>[2x]YEQDKTYKITVLHTNDHHGHFWRNEYGEYGLAAQKTLVDGIRKEVAAEGGSVLLLSGGDINTGVPESDLQDAEPDFRGMNLVGYDAMAIGNHEFDNPLTVLRQQEKWAKFPLLSANIYQKSTGERLFKPWALFKRQDLKIAVIGLTTDDTAKIGNPEYFTDIEFRKPADEAKLVIQELQQTEKPDIIIAATHMGHYDNGEHGSNAPGDVEMARALPAGSLAMIVGGHSQDPVCMAAENKKQVDYVPGTPCKPDQQNGIWIVQAHEWGKYVGRADFEFRNGEMKMVNYQLIPVNLKKKVTWEDGKSERVLYTPEIAENQQMISLLSPFQNKGKAQLEVKIGETNGRLEGDRDKVRFVQTNMGRLILAAQMDRTGADFAVMSGGGIRDSIEAGDISYKNVLKVQPFGNVVVYADMTGKEVIDYLTAVAQMKPDSGAYPQFANVSFVAKDGKLNDLKIKGEPVDPAKTYRMATLNFNATGGDGYPRLDNKPGYVNTGFIDAEVLKA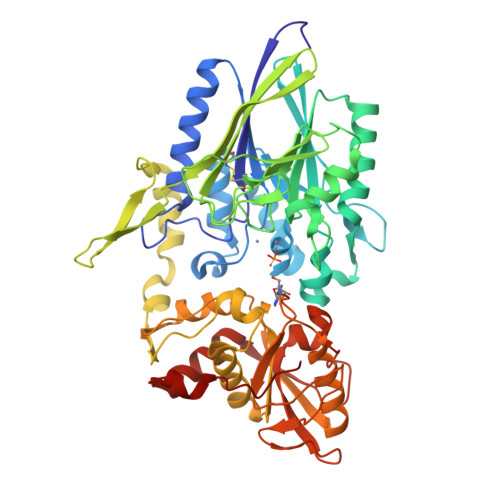YIQKSSPLDVSVYEPKGEVSWQ>GSPNSSVAASTEKTLRLYDRRSIFEAVAQNNCQDLESLL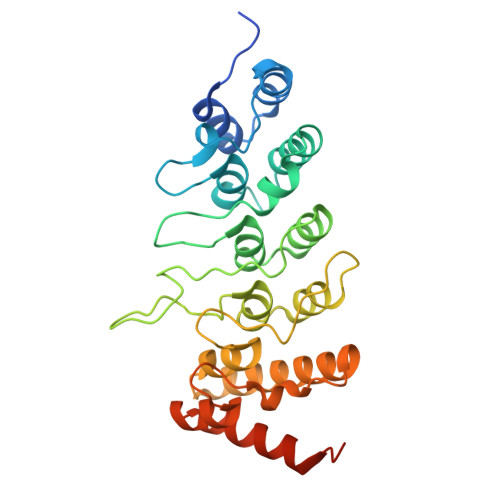LFLQKSKKHLTDNEFKDPETGKTCLLKAMLNLHDGQNTTIPLLLEIARQTDSLKELVNASYTDSYYKGQTALHIAIERRNMALVTLLVENGADVQAAAHGDFFKKTKGRPGFYFGELPLSLAACTNQLGIVKFLLQNSWQTADISARDSVGNTVLHALVEVADNTADNTKFVTSMYNEILMLGAKLHPTLKLEELTNKKGMTPLALAAGTGKIGVLAYILQREIQEPECRHVDSSGRIVTD[6x]>[2x]GPSYHCKTPDCKGWCFFEDDVNEFTCPVCFHVNCLLCKAIHEQMNCKEYQEDLALRAQNDVAARQTTEMLKVMLQQGE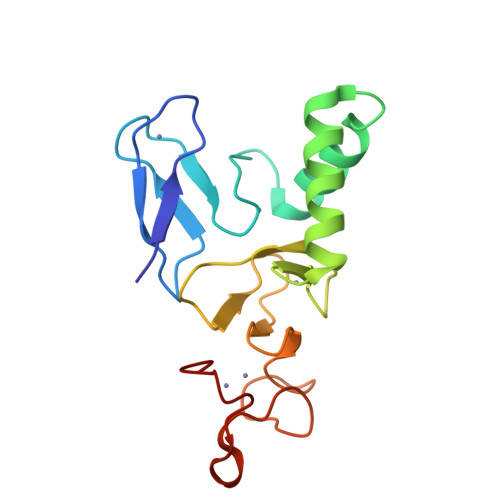AMRCPQCQIVVQKKDGCDWIRCTVCHTEICWVTKGPRWGPGGPGDTSGGCRCRVNGIPCHPSCQNCH> MKLLPESLQQEAATAAVVASWVLWHLDTQLLPTIMREHKLHACWAAAAKRYNEKLFKLNPSYDRVLSLPAVSKNQVLENVFHTAPKAPVEHLEKMVSANSKVYDALNLQSKRVLIWQVKP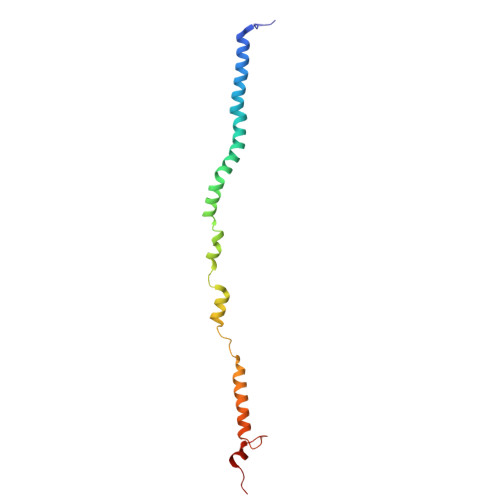ALF> GSHMMTGTIETTGNISAEKGGSIILQCHLSSTTAQVTQVNWEQQDQLLAICNADLGWHISPSFKDRVAPGPGLGLTLQSLTVNDTGEYF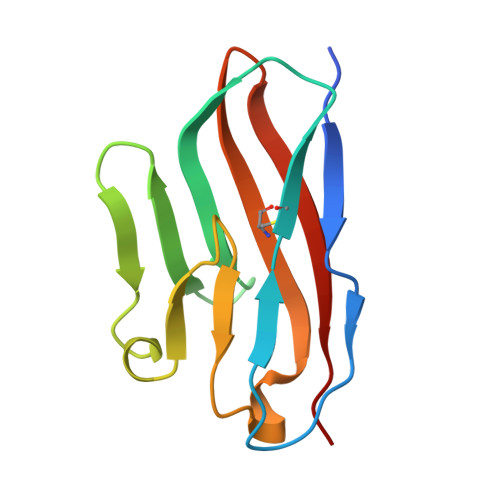CIYHTYPDGTYTGRIFLEVLE> ANLRLSEANSGTYKTFIGRVREELGSETYRL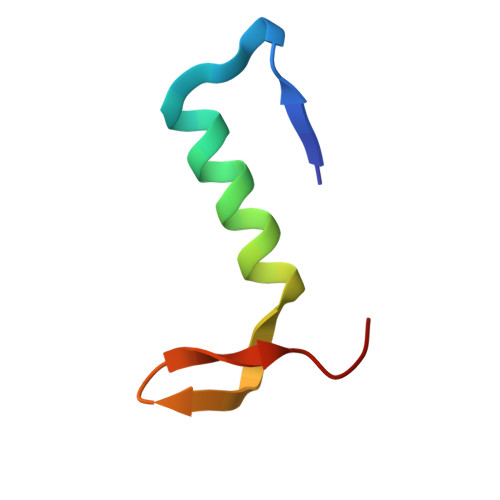YGIPVLKHSL> NLIQFKNMIQCAGTRPWTAYVNYGCYCGKGGSGTPVDELDRCCYTHDNC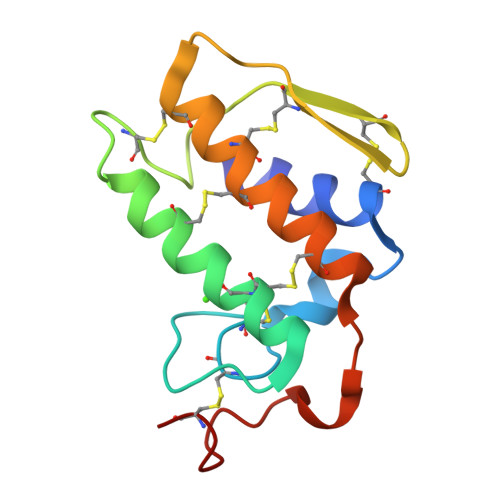YNEAEKIPGCNPNIKTYSYTCTEPNLTCTDTADTCARFLCNCDRTAAICFASAPYNSNNVMISSSTNCQ>[8x]MAKNTSITLGEHFDGFITSQIQSGRYGSASEVIRSALRLLENQETKLQSLRQLLIEGEQSGDADYDLDSFINELDSENIR

ParD2 is the antitoxin component of the parDE2 toxin–antitoxin module from Vibrio cholerae and consists of an ordered DNA-binding domain followed by an intrinsically disordered ParE-neutralizing domain. Like the more intensively studied CcdB, ParE poisons gyrase by stabilizing the so-called cleavable complex between gyrase and DNA. This leads to double-strand breaks, activation of the SOS response and ultimately, if the ParE toxin is not counteracted by the antitoxin ParD, cell death. In analogy to ParD from plasmid RK2 (RKParD; Roberts et al., 1993) and ParD2 from M. tuberculosis, we predicted VcParD2 to be a DNA-binding protein that represses the parDE2 operon.

The VcParD2 sample formed crystals that diffracted to 3.1 Å resolution only after three months. The asymmetric unit contained four dimers of the N-terminal domain of VcParD2 and the corresponding models encompass residues Lys3–Arg51. The N-terminal two and C-terminal 32 residues are not visible in the electron-density map. Dimer formation buries about 1240 Å2 of mainly hydrophobic surface and creates the hydrophobic core of the protein. In the crystal, the VcParD2N dimers are found in a circular arrangement. This results in a torus consisting of eight VcParD22 dimers. The interface formed by adjacent VcParD22 dimers buries roughly 600 Å2. This interface is highly hydrophilic [PISA P(Δi G) value of 0.91] and is dominated by hydrogen bonds and salt bridges, and as such deviates from typical stable oligomerization interfaces. In contrast to SaCopG, VcParD2 does not associate into a helical structure, but forms a closed circle. The dimer–dimer association of VcParD2 is nevertheless very similar to that of SaCopG bound to DNA, suggesting that crystal packing may also reflect associations occurring on the DNA here.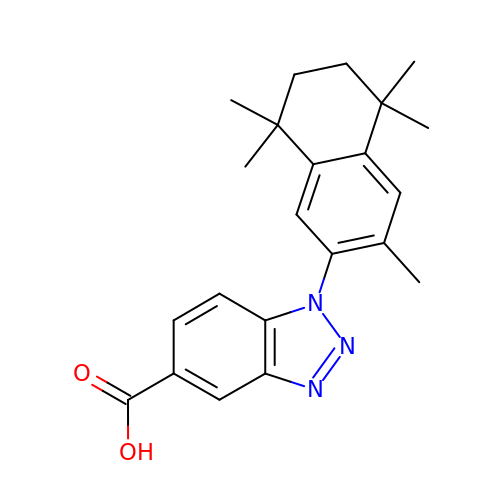1-(3,5,5,8,8-pentamethyl-6,7-dihydronaphthalen-2-yl)benzotriazole-5-carboxylic acid | C22 H25 N3 O2 | QSRQAKVNYDAVIT-UHFFFAOYSA-N> MAAIGRGRSLKNLRVRGRNDSGEENVPLDLTREPSDNLREILQNVARLQGVSNMRKLGHLNNFTKLLCDIGHSEEKLGFHYEDIIICLRLALLNEAKEVRAAGLRALRYLIQDSSILQKVLKLKVDYLIARCIDIQQSNEVERTQALRLVRKMITVNASLFPSSVTNSLIAVGNDGLQERDRMVRACIAIICELALQNPEVVALRGGLNTILKNVIDCQLSRINEALITTILHLLNHPKTRQYVRADVE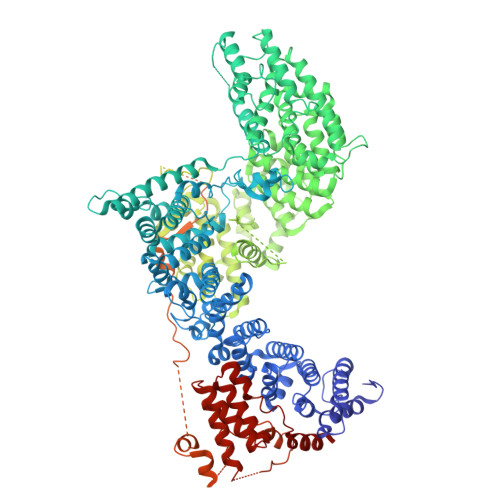LERILAPYTDFHYRHSPDTAEGQLKEDREARFLASKMGIIATFRSWAGIINLCKPGNSGIQSLIGVLCIPNMEIRRGLLEVLYDIFRLPLPVVTEEFIEALLSVDPGRFQDSWRLSDGFVAAEAKTILPHRARSRPDLMDNYLALILSAFIRNGLLEGLVEVITNSDDHISVRATILLGELLHMANTILPHSHSHHLHCLPTLMNMAASFDIPKEKRLRASAALNCLKRFHEMKKRGPKPYSLHLDHIIQKAIATHQKRDQYLRVQKDIFILKDTEEALLINLRDSQVLQHKENLEWNWNLIGTILKWPNVNLRNYKDEQLHRFVRRLLYFYKPSSKLYANLDLDFAKAKQLTVVGCQFTEFLLESEEDGQGYLEDLVKDIVQWLNASSGMKPERSLQNNGLLTTLSQHYFLFIGTLSCHPHGVKMLEKCSVFQCLLNLCSLKNQDHLLKLTVSSLDYSRDGLARVILSKILTAATDACRLYATKHLRVLLRANVEFFNNWGIELLVTQLHDKNKTISSEALDILDEACEDKANLHALIQMKPALSHLGDKGLLLLLRFLSIPKGFSYLNERGYVAKQLEKWHREYNSKYVDLIEEQLNEALTTYRKPVDGDNYVRRSNQRLQRPHVYLPIHLYGQLVHHKTGCHLLEVQNIITELCRNVRTPDLDKWEEIKKLKASLWALGNIGSSNWGLNLLQEENVIPDILKLAKQCEVLSIRGTCVYVLGLIAKTKQGCDILKCHNWDAVRHSRKHLWPVVPDDVEQLCNELSSIPSTLSLNSESTSSRHNSESESVPSSMFILEDDRFGSSSTSTFFLDINEDTEPTFYDRSGPIKDKNSFPFFASSKLVKNRILNSLTLPNKKHRSSSDPKGGKLSSESKTSNRRIRTLTEPSVDFNHSDDFTPISTVQKTLQLETSFMGNKHIEDTGSTPSIGENDLKFTKNFGTENHRENTSRERLVVESSTSSHMKIRSQSFNTDTTTSGISSMSSSPSRETVGVDATTMDTDCGSMSTVVSTKTIKTSHYLTPQSNHLSLSKSNSVSLVPPGSSHTLPRRAQSLKAPSIATIKSLADCNFSYTSSRDAFGYATLKRLQQQRMHPSLSHSEALASPAKDVLFTDTITMKANSFESRLTPSRFMKALSYASLDKEDLLSPINQNTLQRSSSVRSMVSSATYGGSDDYIGLALPVDINDIFQVKDIPYFQTKNIPPHDDRGARAFAHDAGGLPSGTGGLVKNSFHLLRQQMSLTEIMNSIHSDASLFLESTEDTGLQEHTDDNCLYCVCIEILGFQPSNQLSAICSHSDFQDIPYSDWCEQTIHNPLEVVPSKFSGISGCSDGVSQEGSASSTKSTELLLGVKTIPDDTPMCRILLRKEVLRLVINLSSSVSTKCHETGLLTIKEKYPQTFDDICLYSEVSHLLSHCTFRLPCRRFIQELFQDVQFLQMHEEAEAVLATPPKQPIVDTSAES> GHMHDCHQVTVSRDVTLQNKERHDCNQVCASIDKETENKLNTDIIPRLTRYMSVKGNSIIARVQQSNSDPKCSCTWRAIIWRVYKAYDENSLNVALHVSHPNQQIGENPDWSLVISNPNVHCLKH

The Dothideomycete Leptosphaeria maculans, causal agent of oilseed rape stem canker or blackleg disease, is one of the fungal pathogens in which suppression of ETI by the presence of an AVR gene has been demonstrated. Among them, AvrLm4-7 suppresses Rlm3-mediated resistance triggered by AvrLm3 and Rlm9-mediated resistance triggered by AvrLm5-9. Surprisingly, despite low sequence similarity, AvrLm5-9 and AvrLm3 are structural analogues of AvrLm4-7, sharing an anti-parallel β-sheet covered by α-helices. Structure-informed sequence database searches identified a larger number of putative structural analogues among L. maculans effector candidates, including the AVR effector AvrLmS-Lep2, all produced during the early stages of oilseed rape infection, as well as among effector candidates from other phytopathogenic fungi. These structural analogues are named LARS (for Leptosphaeria AviRulence and Suppressing) effectors.

The structure of AvrLm5-9 was solved using iodine single wavelength anomalous diffusion (SAD) signal from a derivative crystal and then refined at 2.14 Å resolution using native data. The structure of AvrLm5-9 consists of a central β-sheet made of three anti-parallel β-strands. An elongated peptide (residues 54 to 64) runs anti-parallel to β-strand 2, but only establishes a few main-chain H-bonds, and therefore is not categorized as a β-strand. One face of the β-sheet is covered by the long connections between the stands. The connection between the β1 and β2 strands is a curved α-helix and the connection between the β3 and β4 strands contains a shorter helix surrounded by two irregular peptide loops. AvrLm5-9 has three disulfide bridges, which are C3-C119, C22-C69 and C26-C71, named SS1, SS2 and SS3, respectively, according to protein numeration without the signal peptide or C22-C138, C41-C88 and C45-C90 according to protein numeration with the signal peptide. The SS1 bridge knits the N- and C-termini together, while the other two disulfide bridges fix the long helix onto the β-sheet. The two last polymorphic residues were mapped onto the AvrLm5-9 3D structure. The mutation leading to virulence towards Rlm9 is situated in the middle of the long helix, and the mutation having no effect on the interaction with Rlm9 and Rlm5 is in a loop connecting β1 and β2. Neither mutation is expected to perturb the 3D structure.> SVYPKALRDEYIMSKTLGSGACGEVKLAFERKTCKKVAIKIISKRKFAIGSAREADPALNVETEIEILKKLNHPCIIKIKNFFDAEDYYIVLELMEGGELFDKVVGNKRLKEATCKLYFYQMLLAVQYLHENGIIHRDLKPENVLLSSQEEDCLIKITDFGHSKILGETSLMRTLCGTPTYLAPEVLVSVGTAGYNRAVDCWSLGVILFICLSGYPPFSEHRTQVSLKDQITSGKYNFIPEVWAE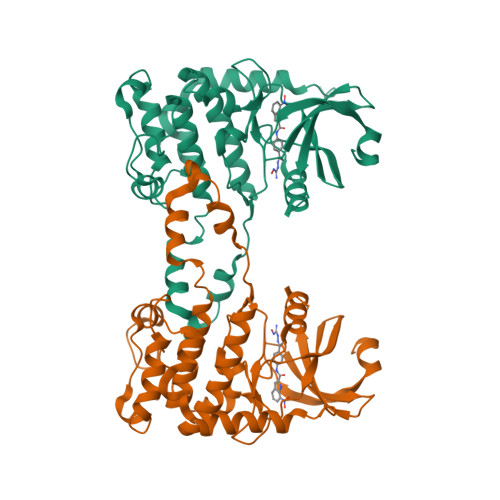VSEKALDLVKKLLVVDPKARFTTEEALRHPWLQDEDMKRKFQDLLSEENESTALPQVLAQPSTSRKRPREGEAEGAE> MATETATRDQLTKEAFQNPDNQKVNIDELGNAIPSGVLKDDVVANIEEQAK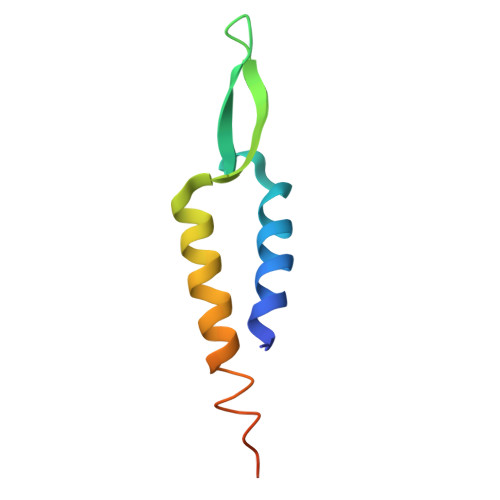AAGEEAKQQAIENLEHHHHHH>[2x]MSLKKY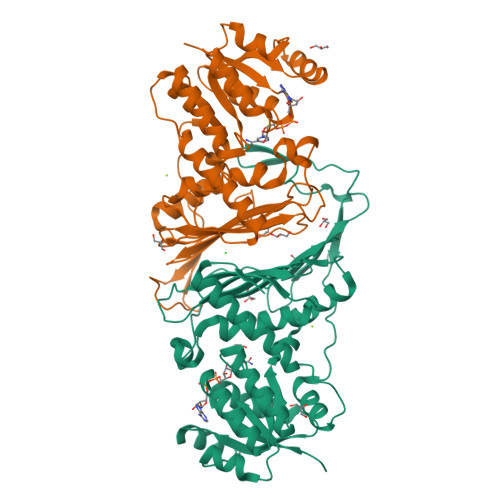QLVIVGYGGMGSYHVTLASAADNLEVHGVFDILAEKREAAAQKGLKIYESYEAVLADEKVDAVLIATPNDSHKELAISALEAGKHVVCEKPVTMTSEDLLAIMDVAKRVNKHFMVHQNRRWDEDFLIIKEMFEQKTIGEMFHLESRVHGANGIPGDWRHLKAHGGGMVLDWGVHLLDQLLFLVDSNVKSVSANLSFALGDEVDDGFVTFITFENGITAQIEVGTTNFIKLPRWYVKGTEGTGIIHDWDLSGEIVKPTALAKTSEPTPIKAGQGLTKTMAPPSEEATNTLSLPAPAKLAPSFYNNFVDVLNNTSEPIVQNEEVYQVLKLIEAIFEAAETNRTVHSIEGHHHHHH>[2x]VNTIIYNVGSTTISKYATFLNDLRNEAKDPSLKCYGIPMLP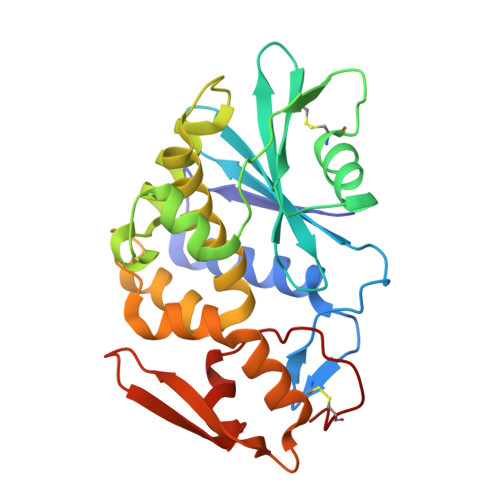NTNTNPKYVLVELQGSNKKTITLMLRRNNLYVMGYSDPFETNKCRYHIFNDISGTERQDVETTLCPNANSRVSKNINFDSRYPTLESKAGVKSRSQVQLGIQILDSNIGKISGVMSFTEKTEAEFLLVAIQMVSEAARFKYIENQVKTNFNRAFNPNPKVLNLQETWGKISTAIHDAKNGVLPKPLELVDASGAKWIVLRVDEIKPDVALLNYVGGSCQTT3-(phosphonooxy)propanoic acid | C3 H7 O6 P | 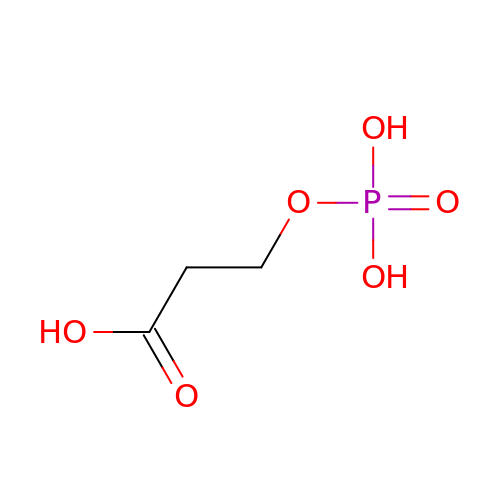QMMAAPSPIPKBBV-UHFFFAOYSA-N>MMELIRIAMKKDLENDNSLMNKWATVAGLKNPNPLYDFLNHDGKTFNEFSSIVNIVKSQYPDREYELMKDYCLNLDVKTKAARSALEYADANMFFEIEDVLIDSMISCSNMKSKEYGKVYKIHRELSNSVITEFEAVKRLGKLNIKTPEMNSFSRLLLLYHYLSTGNFSPMAQLIKQIDLSEISENMYIRNTYQTRVHVLMSNIKLNENSLEECREYSKKALESTNILRFQVFSYLTIGNSLLFSNYELAQENFLKGLSISVQNENYNMIFQQALCFLNNVWRKENKWINFESDSIMDLQEQAHCFINFNENSKAKEVLDKLDLLVHNDNELAMHYYLKGRLEQNKACFYSSIEYFKKSNDKFLIRLPLLELQKMGENQKLLELLLLLEHHHHHH[2x];>GMPRGA[2x]

Recently, in Bacillus phages, a peptide communication system named the arbitrium system was identified that plays an essential role in lysis–lysogeny decisions during infection of Bacillus host cells. This system requires the arbitrium hexapeptide to bind to its cellular receptor AimR to regulate transcription of the lysogeny negative regulator gene aimX. AimR is composed of two domains, a N-terminal domain that is responsible for DNA binding and a C-terminal domain that specifically recognizes the arbitrium peptide. The overall structure of AimR is similar to that of RRNPP family proteins.

In our previous reported structures of apo- and peptide-bound AimR, we were unable to trace the N-terminal DBD structure due to the poor electronic densities. In this study, we reoptimized the crystals and collected new datasets for AimR with or without the peptide. Finally, we traced the density of the DBD for AimR with or without the peptide. In the apo- and peptide-bound form, the AimR dimer exhibits an inverted trapezoid-like fold. The last C-terminal capping helices from two AimR molecules undergo dimerization via a network of van der Waals interactions. The distance between the two aspartic acid residues in the inner cavity, D15 of AimRA and D15 of AimRB, is approximately 125 Å in apo- or peptide-bound AimR. The C-terminal domain coordinates the arbitrium peptide GMPRGA via its four atypical TPR repeats. The arbitrium peptide enriched the low-FRET species, while the high-FRET population was reduced. Upon peptide binding, AimR is trapped in the open state, and it is difficult to transition to the closed state. In turn, the peptide inhibits AimR binding to the target DNA.>UTCTGCTGCTGAA[4x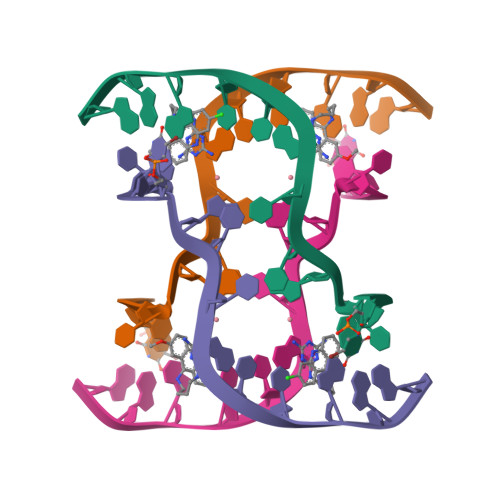]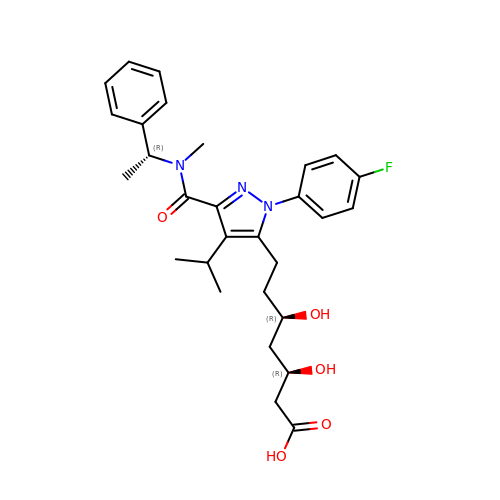(3R,5R)-7-[1-(4-fluorophenyl)-4-(1-methylethyl)-3-{methyl[(1R)-1-phenylethyl]carbamoyl}-1H-pyrazol-5-yl]-3,5-dihydroxyheptanoic acid | C29 H36 F N3 O5 | MPDDTAJMJCESGV-CTUHWIOQSA-N DAUNOMYCIN 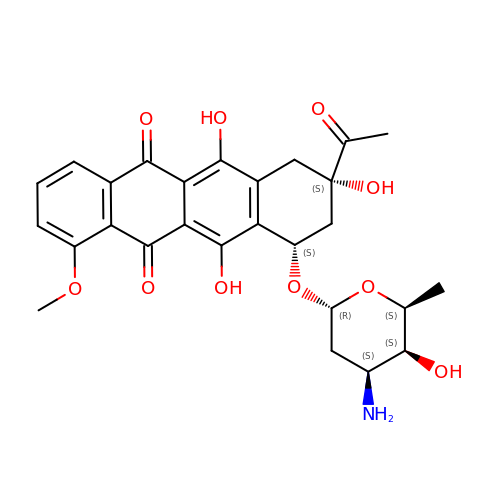| C27 H29 N O10 | STQGQHZAVUOBTE-VGBVRHCVSA-N> TCGGCG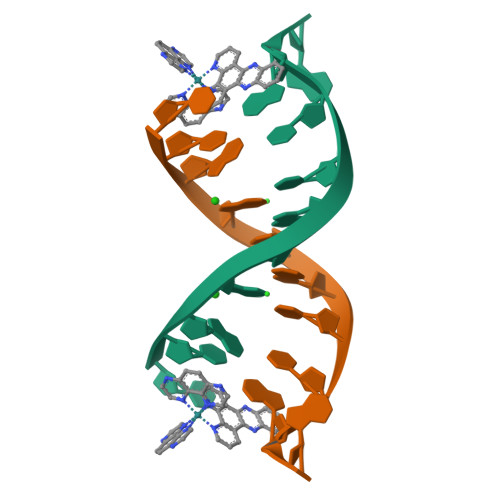CCIA(7R)-2-[(3,5-difluoro-4-hydroxyphenyl)amino]-8-ethyl-7-methyl-5-(prop-2-yn-1-yl)-7,8-dihydropteridin-6(5H)-one 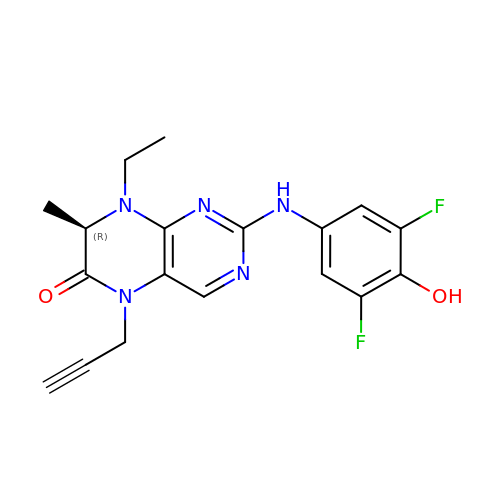| C18 H17 F2 N5 O2 | ZPVLKVQCFYVQDJ-SNVBAGLBSA-N> MHSTNNNSNKRNNEEKHKQPEIDSSANNGEGTSGTRAQTVGDTATEAGVRNETKAGASTRRQTDGTGLSGTNAKIATASSARQTDVEKPADVTFT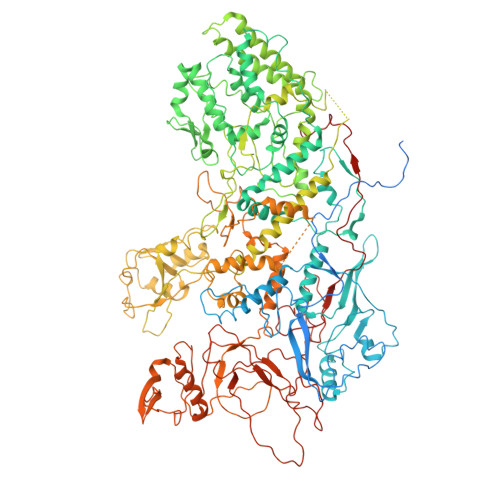IENVDDVGIMQQKKPPTVVQSRTDVFNEQFANEALHPMTKVIFNGLDVNTEVQPLSDDFKQISDPKGYLTYSVKYEDQFTKKDKLRASEADDRIVGPTVNLFKYGAAVVNIDLNRDFFDTATGIDLTKGIPLVQDLLVPIGVTAGAEQSAEYVSGLLMVLFKVMTDNRLVIVGETTTPMSNTLSTVVNNVLRTTYHNNVGVNPALLRDFTQVNWLNRDITNMLQQAGTKYGLGLTETRLDYVRLVKTIVGHALNIDHFAASVLNINLRALMEANVTADDRIKALQAHSMISTQFHGPNQGALRPELAFDHDHIIRCLMLAAANYPRLEGIIVQINTGYVASANVIRPVSEKRYFPENLEQNQSAARLVSAVKARASEADISSIHLAIAREVSPMFNVHELKKIAESFEDPSSIVVVLEFILFALFFPTEFNRIKGDIQNVLLLFFSRWYPVEYGIFIQRGATYTINAAGEFEFSGRNEKWDQSLYLSEHFPALFSDVPLAGANTIIAIMRLFTPQGFLRTDDLAIAANFPRASRNPQTYIPYTNQRGTVTNEFASRFRTIVATLANVVNERAVQDDMQKATRSCTKQWLRHLETQFDNIAVAHTDHLSVVYATMSNFMLNFTNNFSGNHATFKPDQYVITSPEGSYKPIIERQGETVDGLTIIDTSIVWPILCQCTYPLVRQSGKGVDAVSIMEEIVYPDPSTTLSQSLSVAQVLSKLTLPDAFINMILSGGDSVVMRTYQTEADDDLDEGIRMTTYDQYLSHIRERLHITNVPDPIYITGASTPDQIAASVQATHVAVVLYQSGVINGSASTYLRENEVLVVMPDYYDVVSRFANANLQMNNNRYHESVLEIADIFDQADFIQTSDAVRQLRALMPTLSTSQIRHAIERIAQITDVDSTDYGKLTLRFLGTLTRSLKMQNAQIRRIRPDGTVLRYDDQIDIEAFRWSRYFLDELRLRRLSVGLRLITNPRIARRFDGVRIMYLTDDDPDPDFVPDVPEGYVAVQYAHRLFSSSLANKRNRVTYTHPPTGMAYPSPTGRPHVHMTINERAGMSKLVADNIIASVIKSNWVVDIHDIEYTAEVMTPSEGYTQHVDAESIMTAPKGKLFHLQFMDGLLRPEPSAFDPPASGEDMRLIYPLQPISVARSMRAIVNHNEVDRPRGAVAPSSYEMDTGTLSRNGDLLYSPVANGQVGIPKLEVDHISFSNVVSMMTANIRTGDDMAVERVNPDDVRAINIRNA>MADADEGFGLAHTPLEPDAKDLPCDSKPESALGAPSKSPSSPQAAFTQQGMEGIKVFLHERELWLKFHEVGTEMIITKAGRRMFPSYKVKVTGLNPKTKYILLMDIVPADDHRYKFADNKWSVTGKAEPAMPGRLYVHPDSPATGAHWM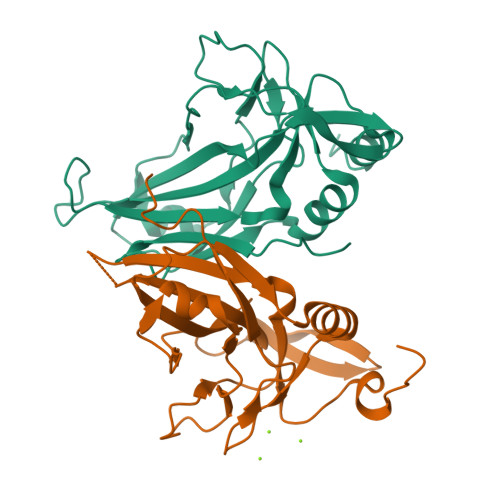RQLVSFQKLKLTNNHLDPFGHIILNSMHKYQPRLHIVKADENNGFGSKNTAFCTHVFPETAFIAVTSYQNHKITQLKIENNPFAKGFRGS[2x]> MGSSHHHHHHSQDPAGPIVELDAQGNEIYYRTLSEQHLEILRNNFEVPPTSETFISPLQSY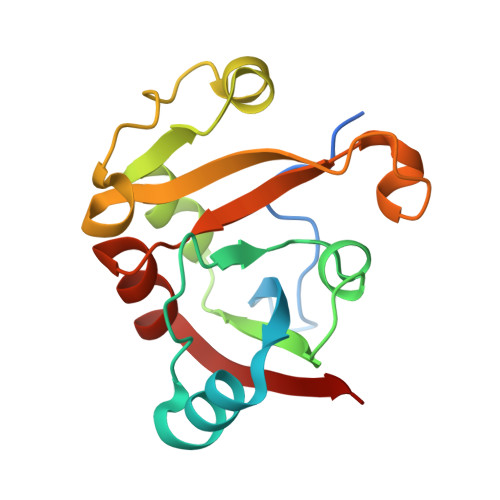SQEYDGKLVRLTASPGTMNELSKIGVTANSGTGLLLPDLPPARKGWKQNNALFKLEALKKPTINEGGGVINTGLGDGKALEIFNKNLIDFEVID> MSEEKTYKRVEQDDPVPELDIKQGPVRPFIVTDPSAELASLRTMVTLKEKLLVACLAVFTAVIRLHGLAWPDSVVFDEVHFGGFASQYIRGTYFMDVHPPLAKMLYAGVASLGGFQGDFDFENIGDSFPSTTPYVLMRFFSASLGALTVILMYMTLRYSGVRMWVALMSAICFAVENSYVTISRYILLDAPLMFFIAAAVYSFKKYEMYPANSLNAYKSLLATGIALGMASSSKWVGLFTVTWVGLLCIWRLWFMIGDLTKSSKSIFKVAFAKLAFLLGVPFALYLVFFYIHFQSLTLDGDGASFFSPEFRSTLKNNKIPQNVVADVGIGSIISLRHLSTMGGYLHSHSHNYPAGSEQQQSTLYPHMDANNDWLLELYNAPGESLTTFQNLTDGTKVRLFHTVTRCRLHSHDHKPPVSESSDWQKEVSCYGYSGFDGDANDDWVVEIDKKNSAPGVAQERVIALDTKFRLRHAMTGCYLFSHEVKLPAWGFEQQEVTCASSGRHDLTLWYVENNSNPLLPEDTKRISYKPASFISKFIESHKKMWHINKNLVEPHVYESQPTSWPFLLRGISYWGENNRNVYLLGNAIVWWAVTAFIGIFGLIVITELFSWQLGKPILKDSKVVNFHVQVIHYLLGFAVHYAPSFLMQRQMFLHHYLPAYYFGILALGHALDIIVSYVFRSKRQMGYAVVITFLAASVYFFKSFSPIIYGTPWTQELCQKSQWLSGWDYNCNTYFSSLEEYKNQTLTKRESQPAATSTVEEITIEGDGPSYEDLMNEDGKKIFKDTEGNELDPEVVKKMLEEEGANILKVEKRAVLE;> MSSSSSTGYSKNNAAHIKQENTLRQRESSSISVSEELSSADERDAEDFSKEKPAAQSSLLRLESVVMPVIFTALALFTRMYKIGINNHVVWDEAHFGKFGSYYLRHEFYHDVHPPLGKMLVGLSGYLAGYNGSWDFPSGEIYPDYLDYVKMRLFNASFSALCVPLAYFTAKAIGFSLPTVWLMTVLVLFENSYSTLGRFILLDSMLLFFTVASFFSFVMFHNQRSKPFSRKWWKWLLITGISLGCTISVKMVGLFIITMVGIYTVIDLWTFLADKSMSWKTYINHWLARIFGLIIVPFCIFLLCFKIHFDLLSHSGTG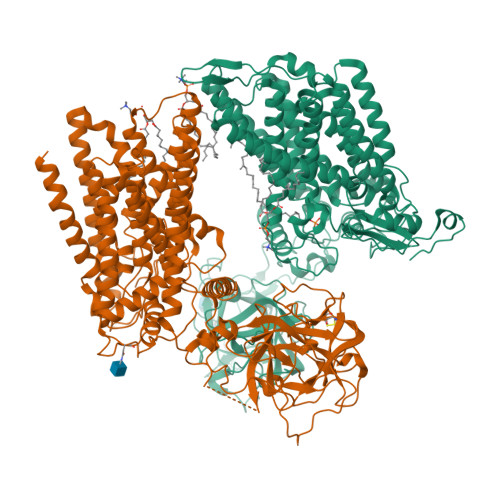DANMPSLFQARLVGSDVGQGPRDIALGSSVVSIKNQALGGSLLHSHIQTYPDGSNQQQVTCYGYKDANNEWFFNRERGLPSWSENETDIEYLKPGTSYRLVHKSTGRNLHTHPVAAPVSKTQWEVSGYGDNVVGDNKDNWVIEIMDQRGDEDPEKLHTLTTSFRIKNLEMGCYLAQTGNSLPEWGFRQQEVVCMKNPFKRDKRTWWNIETHENERLPPRPEDFQYPKTNFLKDFIHLNLAMMATNNALVPDPDKFDYLASSAWQWPTLNVGLRLCGWGDDNPKYFLLGTPASTWASSVAVLAFMATVVILLIRWQRQYVDLRNPSNWNVFLMGGFYPLLAWGLHYMPFVIMSRVTYVHHYLPALYFALIILAYCFDAGLQKWSRSKCGRIMRFVLYAGFMALVIGCFWYFSPISFGMEGPSSNFRYLNWFSTWDIADKQEA Protein A075L is a β‐xylosyltransferase that participates in producing the core of the N‐glycans found in VP54, the major viral capsid protein of Paramecium bursaria chlorella virus‐1 (PBCV‐1). The protein structure shows a typical GT‐B folding, with two Rossmann‐like fold domains, in which the acceptor substrate binds to the N‐terminal region, and the nucleotide‐sugar donor binds to the C‐terminal region. We propose that the catalytic mechanism follows a direct displacement SN2‐like reaction, where Asp73 serves as a catalytic base that deprotonates the incoming nucleophile of the acceptor, facilitating direct displacement of the UDP with the inversion of the anomeric configuration of the acceptor without metal ion dependence, while the interactions with side chains of Arg158 and Arg208 stabilize the developing negative charge. In this context, we herein present the structural and biochemical characterization of A075L, a soluble chlorovirus xylosyltransferase easily produced in E. coli and amenable to large‐scale purification.

The density map of UDP‐α‐D‐Xyl identified the sugar donor in a well‐defined pocket where Asn148 coordinates the uracil moiety, and Arg208 and Arg158 coordinate the phosphate groups. Among the 17 well‐defined direct hydrogen bonds with 1, there are four H‐bonds between A075L and the nucleoside moiety and three specific H‐bonds with the Xyl moiety. Thus, A075L recognizes 1 with very high specificity. First, a double mutant (N148A, R208A), targeting those enzyme residues involved in the interaction with the ribose, the bases, and the phosphate moieties of the donor, was analyzed. In contrast, significant STD signals were observed for the acceptor 6. These results provide support for the proposal that the side chains of Asn148 and Arg208 are key for the binding of the donor, but do not affect the binding of the trisaccharide acceptor. Introduction of point mutations such as N148A and R208A affect the binding of the UDP‐xylose donor, but not the recognition of the acceptors. To understand the details of the glycosyl transfer mechanism, the geometries of A075L in complex with the donor and acceptor were initially superimposed. However, inspection of the superimposed structures showed that the distance between O4 Fuc and C1 Xyl exceeded 3.0 Å, too far for the nucleophilic attack. Additionally, it was deduced that the orientation of the UDP‐α‐D‐Xyl donor with respect to the Fuc moiety in the acceptor was not the proper one for the nucleophilic attack to take place. Hence, we hypothesized that a conformational rearrangement takes place for catalysis to occur.

>[4x]LGSMKLAELTLESDDFITSDKLFNFCKSTIFGAKYVKTDFIKFRQYQYIVSNCGWRDDTDVVFLENTPVLVTGHSDYDISEREIDIIRLPNIRAWFCQNRNIPHPKVISFPLGITNKDEPNSEIHRIIGNTDRILEVSKTPKEIKNLVYMNITVKNFPEERQRIVDLYSDKSWVTIGKGEVSEEGHRKFLEDMYAHKFCFAPRGNGIDTHRLWESLYLRTIPIVKKHIAMEQFTDLPILFVNDWENITEEYLNEQYDIIMAKDWNLDKLKIDYWYQKILEYSQ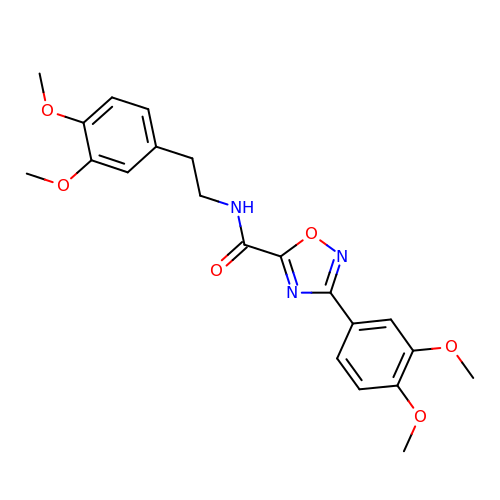3-(3,4-dimethoxyphenyl)-~{N}-[2-(3,4-dimethoxyphenyl)ethyl]-1,2,4-oxadiazole-5-carboxamide | C21 H23 N3 O6 | GVKZOYXTOVFRQE-UHFFFAOYSA-N Encoded by the smallest of the eight viral genome segments, NS1 is a multifunctional RNA-binding protein, which is considered the main weapon of the virus to antagonize the innate immune response of the host and to ensure viral replication in a hostile anti-viral environment. While the effector domain is to some extent dispensable for the biological activities of NS1, the RBD plays an essential role in several activities that require the interaction of NS1 with viral and non-viral RNAs. This is best illustrated by the total loss of pathogenicity conferred by the alanine substitution of Arg38 and Lys41, the two main residues involved in binding of RNAs by NS1.

The X-ray structure of recombinant wild type H7N1 NS1 RBD (residues 1–73) was solved to 1.93 Å resolution. While it is the first structure that is representative of the RBD of allele B-NS1, its organization is identical to that of the other RBD structures available, forming a symmetric C2 homodimer shaped by three interlocking α-helices from each monomer. Helices α1 (residues S3-M24) and α2 (A30 to L50) are oriented in an antiparallel fashion, whereas helix α3 (L54-K70) sits perpendicular to helix α1. The dimerization interface, with an area of 1189Å2, involves 43% of the monomer residues, which are engaged in 15 H-bonds, including 4 salt bridges (PISA server). Three highly conserved residues of α2 helix (F32, R35, and R46) are involved in the stabilization of the dimer, with R35 being engaged in a salt bridge with D12. Invariant residues R35, R37, R38, and K41, which are involved in RNA binding, adopt different conformations when comparing all the apo RBD homodimers. Nonetheless, the RNA binding interface formed by helices α2 and α2* of the homodimer seems to be well preserved on H7N1. This 3D structure also shows several ligands bound to the RBD, originating from the crystallization buffers. Three 1,2-ethanediol and one partial polyethylene glycol molecules have been assigned in a groove formed by helices α3 and α3*. Interestingly, another partial polyethylene glycol molecule is located in a nonpolar pocket found underneath the RNA binding channel at the RBD molecular two-fold axis (between helices α2 and α2*), making an H-bond with the side chain of R46(A).

>GSHMSDSNTITSFQVDCYLWHIRKLLSMRDMCDAPFDDRLRRDQKALKGRGSTLGLDLRVATMEGKKIVEDILKSET[2x]>[4x]GPNTEFALSLLRKNIMTITTSKGEFTGLGIHDRVCVIPTHAQPGDDVLVNGQKIRVKDK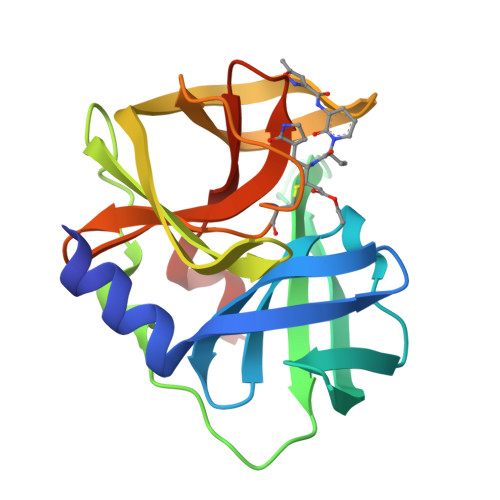YKLVDPENINLELTVLTLDRNEKFRDIRGFISEDLEGVDATLVVHSNNFTNTILEVGPVTMAGLINLSSTPTNRMIRYDYATKTGQCGGVLCATGKIFGIHVGGNGRQGFSAQLKKQYFVEKQ> GSGSGSGMSWIKEGELSLWERFCANIIKAGPMPKHIAFIM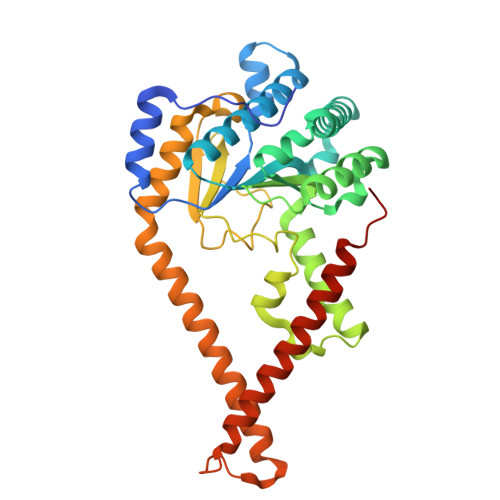DGNRRYAKKCQVERQEGHSQGFNKLAETLRWCLNLGILEVTVYAFSIENFKRSKSEVDGLMDLARQKFSRLMEEKEKLQKHGVCIRVLGDLHLLPLDLQELIAQAVQATKNYNKCFLNVCFAYTSRHEISNAVREMAWGVEQGLLDPSDISESLLDKCLYTNRSPHPDILIRTSGEVRLSDFLLWQTSHSCLVFQPVLWPEYTFWNLFEAILQFQMNHSVLQKARDMYAEERKRQQLERDQATVTEQLLREGLQASGDAQLRRTRLHKLSARREERVQGFLQALELKRADWLARLGTASA> MKIISKEFTVKTRSRFDSIDITEQVSEAIKGINNGIAHVIVKHTTCAIIINEAESGLMKDFLNWAKKLVPPDGEFEHN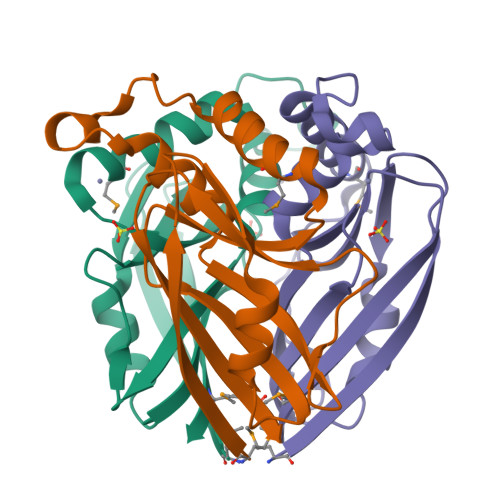IIDNNGHAHVISAIIGNSRVVPIIEGKLDLGTWQRIILLEFDGPRTRTVLVKSMGE> MSKINVNVENVSGVQGFLFHTDGKESYGYRAFINGVEIGIKDIETVQGF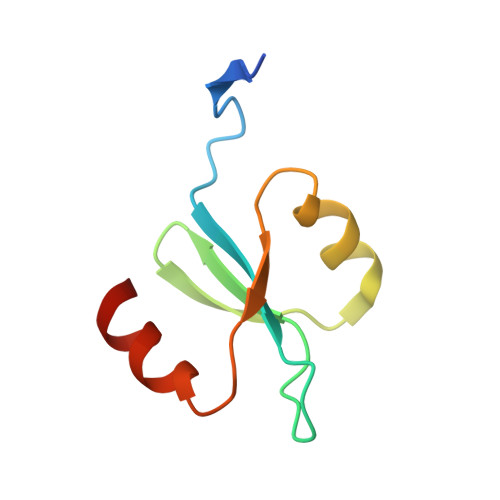QQIIPSINISKSDVEAIRKAMKK> MNYSADSGNTVYVGNIDPRITKEQLYELFIQINPVLRIKYPKDKVLQAYQGYAFIEFYNQGDAQYAIKIMNNTVRLYDRLIKVRQVTNSTGT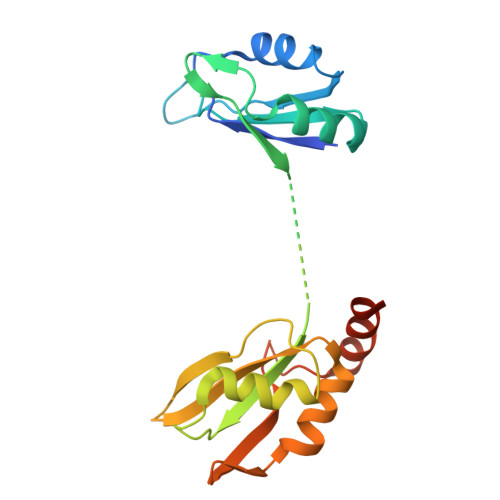TNLPSNISKDMILPIAKLFIKNLADSIDSDQLVKIFNKFGKLIREPEIFYLSNGKLKCAYVYFEDFEKADLAIKSLNNQLVANNRITVDYAFKENGKGNAKYGDDVDRLLNKEALKHNMLK> RVKRTYEVTRQNDNAVRIEPSSLGEEEDKEAKDKNSALQLKRSRYDPNKVFSNTNQGPEKNNLKGEQLGSQKKSSKYDEKITSNNELTTKKGLLGDSENETKYASSNSKFNVEVTHKIKNAKEIDKINRQRMWEEQQLRNAMAGQSDHPDDITLEGSDKYDYVFDTDAMIDYTNEEDDLLPEEKLQYEARLAQALETEEKRILTIQEARKLLPVHQYKDELLQEIKKNQVLIIMGETGSGKTTQLPQYLVEDGFTDQGKLQIAITQPRRVAATSVAARVADEMNVVLGKEVGYQIRFEDKTTPNKTVLKYMTDGMLLREFLTDSKLSKYSCIMIDEAHERTLATDILIGLLKDILPQRPTLKLLISSATMNAKKFSEFFDNCPIFNVPGRRYPVDIHYTLQPEANYIHAAITTIFQIHTTQSLPGDILVFLTGQEEIERTKTKLEEIMSKLGSRTKQMIITPIYANLPQEQQLKIFQPTPENCRKVVLATNIAETSLTIDGIRYVIDPGFVKENSYVPSTGMTQLLTVPCSRASVDQRAGRAGRVGPGKCFRIFTKWSYLHELELMPKPEITRTNLSNTVLLLLSLGVTDLIKFPLMDKPSIPTLRKSLENLYILGALNSKGTITRLGKMMCEFPCEPEFAKVLYTAATHEQCQGVLEECLTIVSM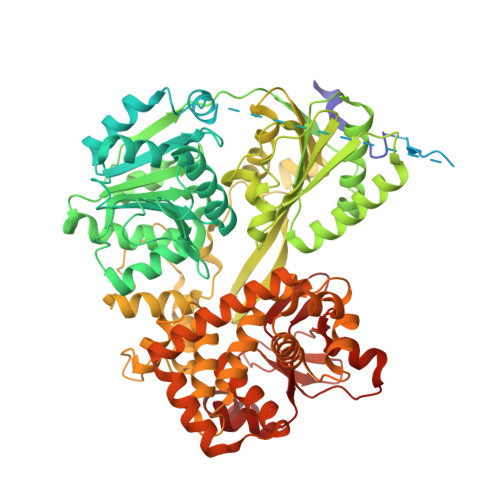LHETPSLFIGQKRDAAASVLSEVESDHILYLEIFNQWRNSKFSRSWCQDHKIQFKTMLRVRNIRNQLFRCSEKVGLVEKNDQARMKIGNIAGYINARITRCFISGFPMNIVQLGPTGYQTMGRSSGGLNVSVHPTSILFVNHKEKAQRPSKYVLYQQLMLTSKEFIRDCLVIPKEEWLIDMVPQIFKDLI>[4x]MSLTASDD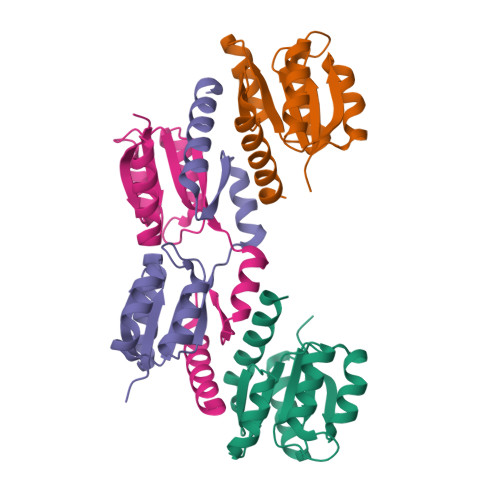LPGVLIVEDGRLAAATLRIQLESLGYDVLGVFDNGEEAVRCAPDLRPDIALVDIMLCGALDGVETAARLAAGCNLPIIFITSSQDVETFQRAKRVNPFGYLAKPVAADTLHRSIEMAIHKKKLEEGHHHHHH> GSASDITQHLNDSGLGPAVE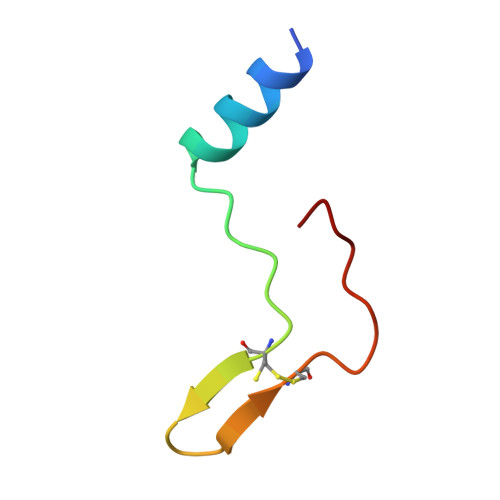CLENLVVGPVCPAAVVAPAV> SLFELGKMILQET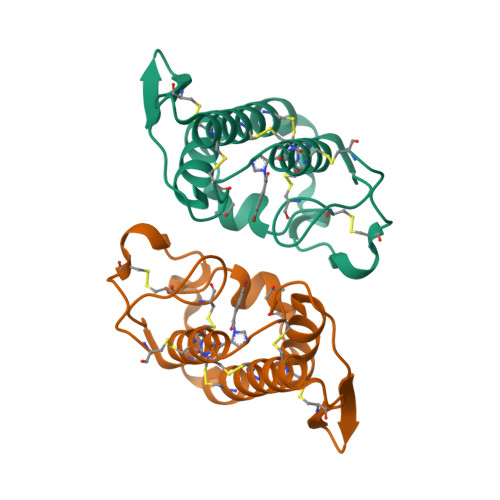GKNPAKSYGAYGCNCGVLGRGKPKDATDRCCYVHKCCYKKLTGCDPKKDRYSYSWKDKTIVCGENNPCLKELCECDKAVAICLRENLGTYNKKYRYHLKPFCKKADPC> PISPIETVPVKLKPGMDGPKVKQWPLTEEKIKALVEICTEMEKEGKISKIGPENPYNTPVFAIKKKDSTKWRKLVDFRELNKRTQDFWEVQLGIPHPAGLKKKKSVTVLDVGDAYFSVPLDEDFRKYTAFTIPSINNETPGIRYQYNVLPQGWKGSPAI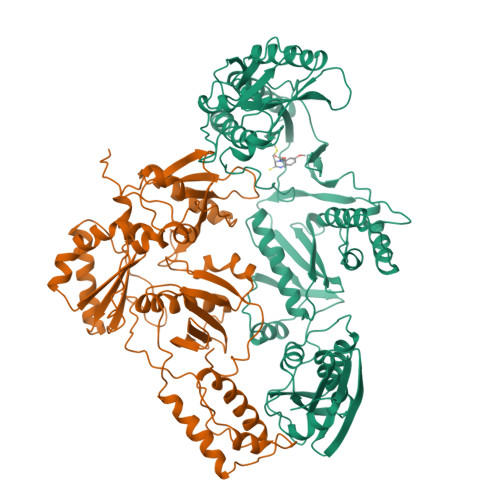FQSSMTKILEPFKKQNPDIVIYQYMDDLLVGSDLEIGQHRTKIEELRQHLLRWGLTTPDKKHQKEPPFLWMGYELHPDKWTVQPIVLPQKDSWTVNDIQKLVGKLNWASQIYPGIKVRQLSKLLRGTKALTEVIPLTEEAELELAENREILKEPVHGVYYDPSKDLIAEIQKQGQGQWTYQIYQEPFKNLKTGKYARMRGAHTNDVKQLTEAVQKITTESIVIWGKTPKFKLPIQKETWETWWTEYWQATWIPEWEFVNTPPLVKLWYQLEKEPIVGAETFYVDGAANRETKLGKAGYVTNKGRQKVVPLTNTTNQKTELQAIYLALQDSGLEVNIVTDSQYALGIIQAQPDKSESELVNQIIEQLIKKEKVYLAWVPAHKGIGGNQQVDKLVSAGIRK;> PISPIETVPVKLKPGMDGPKVKQWPLTEEKIKALVEICTEMEKEGKISKIGPENPYNTPVFAIKKKDSTKWRKLVDFRELNKRTQDFWEVQLGIPHPAGLKKKKSVTVLDVGDAYFSVPLDEDFRKYTAFTIPSINNETPGIRYQYNVLPQGWKGSPAIFQSSMTKILEPFKKQNPDIVIYQYMDDLLVGSDLEIGQHRTKIEELRQHLLRWGLTTPDKKHQKEPPFLWMGYELHPDKWTVEPIVLPEKDSWTVNDIQKLVGKLNWASQIYPGIKVRALSKLLRGTKALTEVIPLTEEAELELAENREILKEPVHGVYYDPSKDLIAEIQKQGQGQWTYQIYQEPFKNLKTGKYARMRGAHTNDVKQLTEAVQKITTESIVIWGKTPKFKLPIQKETWETWWTEYWQATWIPEWEFVNTPPLVKLWYQLE> SMDRRFYGKIVIKGKIKAVTGLHIGSQRDISEIGGIDNP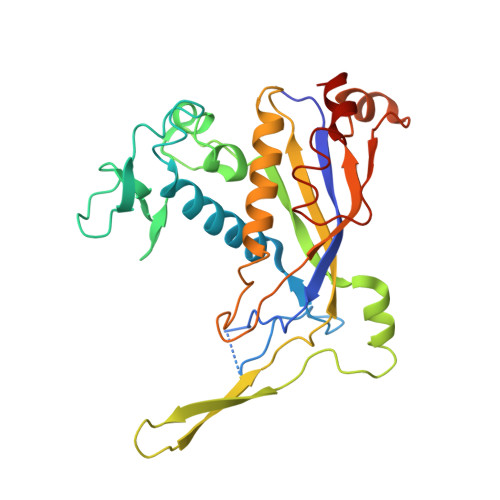VIKDPHTGLPYIPGSSLKGRLRSLFEILVNSRLGEWREKYPSLANYSPGSCRPDNQENCGKFFNRKINRGWIHVCPDYETALACPVCRLFGASGKESNFPSRIIVRDAFLTKEWEEKWRAGEAITEAKIEVGIDRVTSQANPRTNERVVAGAEFEFEIIYNVENTTHWRDDIKNLLTAMALLEDSYLGGSGSRGYGKVKFIFDSFEFRPLDYYRTGKDEDIVSIDAREKSVSDILSGFDSLFSEVEGKLEAG> MNDIAHNLAQVRDKISAAATRCGRSPEEITLLAVSATKPASAIAEAIDAGQRQFGENYVQEGVDKIRHFQELGVTGLEWHFIGPLQSNKSRLVAEHFDWCHTIDRLRIATRLNDQRPAELPPLNVLIQINISDENSASGIQLAELDELAAAVAELPRLRLRGLMAIPAPESEYVRQFEVARQMAVAFAGLKTRYPHIDTLSLGMSDDMEAAIAAGSTMVRIGTAIFGARDYSKK

The pyridoxal 5′‐phosphate (PLP) homeostasis protein (PLPHP) is a ubiquitous member of the COG0325 family with apparently no catalytic activity. Although the actual cellular role of this protein is unknown, it has been observed that mutations of the PLPHP encoding gene affect the activity of PLP‐dependent enzymes, B6 vitamers and amino acid levels. Here we report a detailed characterization of the Escherichia coli ortholog of PLPHP (YggS) with respect to its PLP binding and transfer properties, stability, and structure. YggS binds PLP very tightly and is able to slowly transfer it to a model PLP‐dependent enzyme, serine hydroxymethyltransferase.

We serendipitously discovered that the K36A variant of YggS, affecting the lysine residue that binds PLP at the active site, is able to bind PLP covalently. This observation led us to recognize that a number of lysine residues, located at the entrance of the active site, can replace Lys36 in its PLP binding role.>[2x]MGSSHHHHHHSGLVPRGSHMATPPKRSSPSFSASSEGTRIKKISIEGNIAAGKSTFVNILK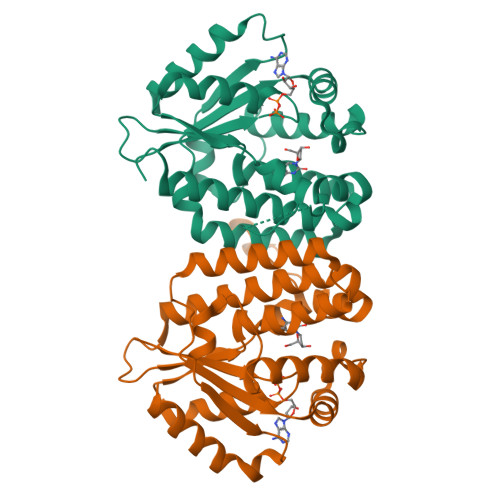QLSEDWEVVPEPVARWSNVQSTQDEFEELTMSQKNGGNVLQMMYEKPERWSFTFQTYACLSRIRAQLASLNGKLKDAEKPVLFFERSVYSDRYIFASNLYESESMNETEWTIYQDWHDWMNNQFGQSLELDGIIYLQATPETCLHRIYLRGRNEEQGIPLEYLEKLHYKHESWLLHRTLKTNFDYLQEVPILTLDVNEDFKDKYESLVEKVKEFLSTL> GRDGNNLNNPVLLLDTFDFGPREDNWFFYPGGNIGLYCPYSSKGAPEEDSAMVFVSNEVGEHSITTRDLSVNENTIIQFEINVGCSTDSSSADPVRLEFSRDFGATWH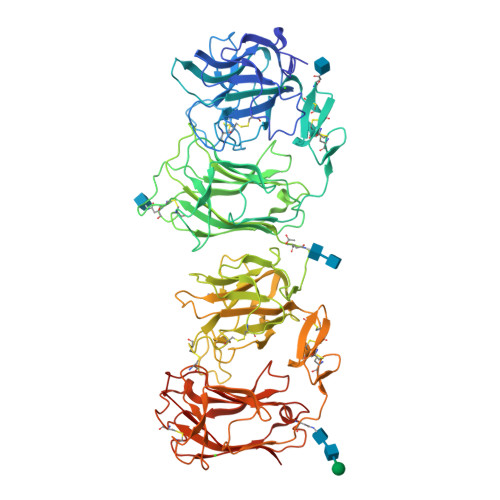LLLPLCYHSSSLVSSLCSTEHHPSSTYYAGTTQGWRREVVHFGKLHLCGSVRFRWYQGFYPAGSQPVTWAIDNVYIGPQCEEMCYGHGSCINGTKCICDPGYSGPTCKISTKNPDFLKDDFEGQLESDRFLLMSGGKPSRKCGILSSGNNLFFNEDGLRMLVTRDLDLSHARFVQFFMRLGCGKGVPDPRSQPVLLQYSLNGGLSWSLLQEFLFSNSSNVGRYIALEMPLKARSGSTRLRWWQPSENGHFYSPWVIDQILIGGNISGNTVLEDDFSTLDSRKWLLHPGGTKMPVCGSTGDALVFIEKASTRYVVTTDIAVNEDSFLQIDFAASCSVTDSCYAIELEYSVDLGLSWHPLVRDCLPTNVECSRYHLQRILVSDTFNKWTRITLPLPSYTRSQATRFRWHQPAPFDKQQTWAIDNVYIGDGCLDMCSGHGRCVQGSCVCDEQWGGLYCDEPETSLPTQLKDNFNRAPSNQNWLTVSGGKLSTVCGAVASGLALHFSGGCSRLLVTVDLNLTNAEFIQFYFMYGCLITPSNRNQGVLLEYSVNGGITWNLLMEIFYDQYSKPGFVNILLPPDAKEIATRFRWWQPRHDGLDQNDWAIDNVLISRLENLYFQ> SNAMKDPLLNSLIYVSRYYGLANSPEALVNGLPLSDGKLTPFLLPRAAERAGLVAKENRAELEKISSLILPAILVLKGGDSCVLNSINMETRE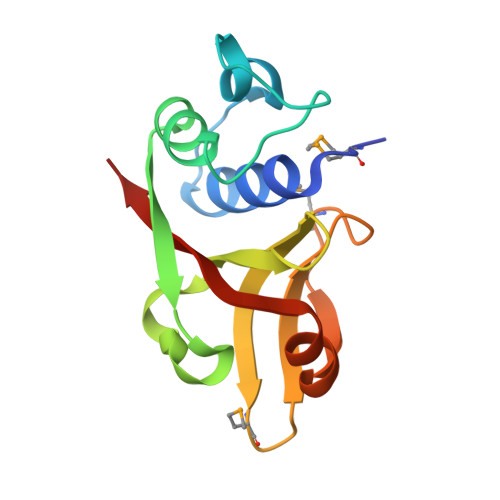AEVTTLESGMVPISIPLEDLLEQYTGRYFLVKKQFR> HHHHHHENLYFQGMSFDNYLVPTVIEQSGRG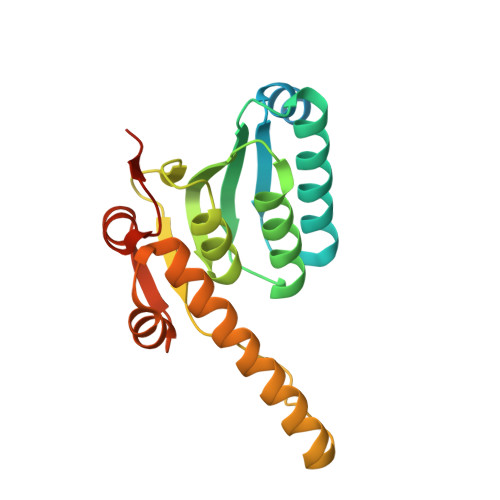ERAFDIYSRLLKERIVFLVGPVTDESANLVVAQLLFLESENPDKDIFFYINSPGGSVTAGMSIYDTMNFIKPDVSTLCLGQAASMGAFLLSAGEKGKRFALPNSRIMIHQPLISGGLGGQASDIEIHARELLKIKEKLNRLMAKHCDRDLADLERDTDRDNFMSAEEAKEYGLIDQILENRASLRL>[10x]GSHMNTNMVASELGVSAKTVQRWVKQLNLPAERNELGHYSFTAEDVKVLKSV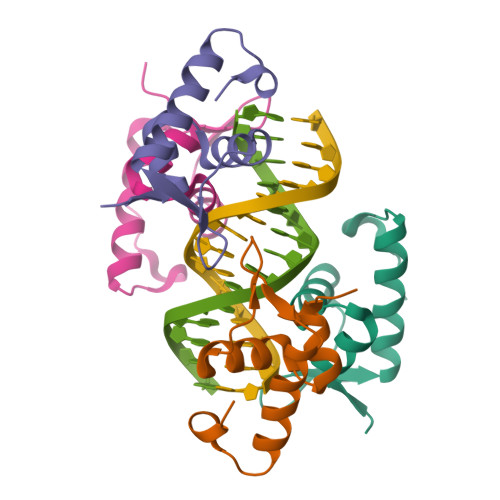KKQISEGTAIQDIHLPK>ADQPIDADVTVIGSGPGGYVAAIKAAQLGFKTVCIEKNETLGGTCLNVGCIPSKALLNNSHYYHMAHGTDFASRGIEMSEVRLNLDKMMEQKSTAVKALTGGIAHLFKQNKVVHVNGYGKITGKNQVTATKADGGTQVIDTKNILIATGSEVTPFPGITIDEDTIVSSTGALSLKKVPEKMVVIGAGVIGVELGSVWQRLGADVTAVEFLGHVGGVGIDMEISKNFQRILQKQGFKFKLNTKVTGATKKSDGKIDVSIEAASGGKAEVITCDVLLVCIGRRPFTKNLGLEELGIELDPRGRIPVNTRFQTKIPNIYAIGDVV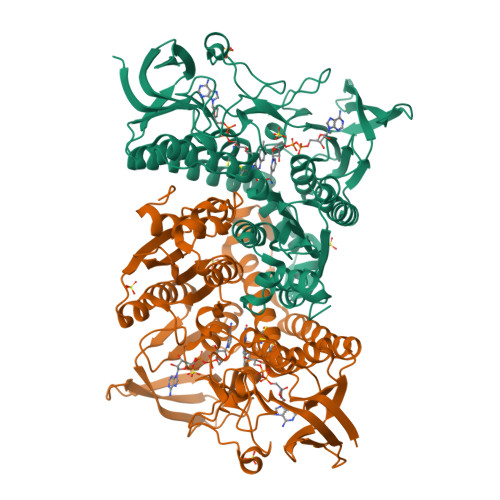AGPMLAHKAEDEGIICVEGMAGGAVHIDYNCVPSVIYTHPEVAWVGKSEEQLKEEGIEYKVGKFPFAANSRAKTNADTDGMVKILGQKSTDRVLGAHILGPGAGEMVNEAALALEYGASCEDIARVCHAHPTLSEAFREANLAASFGKSINF[8x]>MNEALDDIDRILVRELAADGRATLSELATRAGLSVSAVQSRVRRLESRGVVQGYSARINPEAVGHLLSAFVAITPLDPSQPDDAPARLEHIEEVESCYSVAGEESYVLLVRVASARALEDLLQRIRTTANVRTRS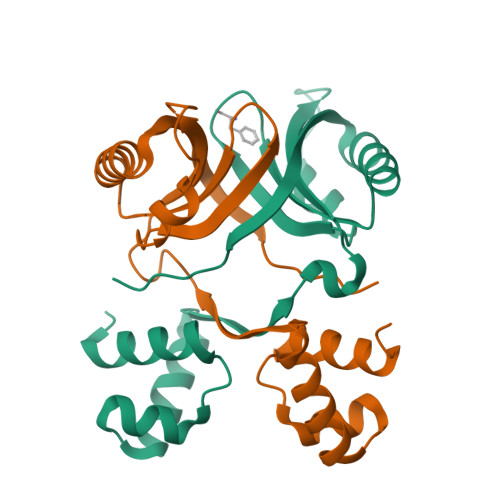TIILNTFYSDRQHIP[2x]> GHHHHHHMIEWIIRRSVANRFLVLMGALFLSIWGTWTIINTPVDALPDLSDVQVIIKTSYPGQAPQIVENQVTYPLTTTMLSVPGAKTVRGFSQFGDSYVYVIFEDGTDPYWARSRVLEYLNQVQGKLPAGVSAELGPDATGVGWIYEYALVDRSGKHDLADLRSLQDWFLKYELKTIPDVAEVASVGGVVKEYQVVIDPQRLAQYGISLAEVKSALDASNQEAGGSSIELAEAEYMVRASGYLQTLDDFNHIVLKASENGVPVYLRDVAKVQIGPEMRRGIAELNGEGEVAGGVVILRSGKNAREVIAAVKDKLETLKSSLPEGVEIVTTYDRSQLIDRAIDNLSGKLLEEFIVVAVVCALFLWHVRSALVAIISLPLGLCIAFIVMHFQGLNANIMSLGGIAIAVGAMVDAAIVMIENAHKRLEEWQHQHPDATLDNKTRWQVITDASVEVGPALFISLLIITLSFIPIFTLEGQEGRLFGPLAFTKTYAMAGAALLAIVVIPILMGYWIRGKIPPESSNPLNRFLIRVYHPLLLKVLHWPKTTLLVAALSVLTVLWPLNKVGGEFLPQINEGDLLYMPSTLPGISAAEAASMLQKTDKLIMSVPEVARVFGKTGKAETATDSAPLEMVETTIQLKPQEQWRPGMTMDKIIEELDNTVRLPGLANLWVPPIRNRIDMLSTGIKSPIGIKVSGTVLADIDAMAEQIEEVARTVPGVASALAERLEGGRYINVEINREKAARYGMTVADVQLFVTSAVGGAMVGETVEGIARYPINLRYPQSWRDSPQALRQLPILTPMKQQITLADVADIKVSTGPSMLKTENARPTSWIYIDA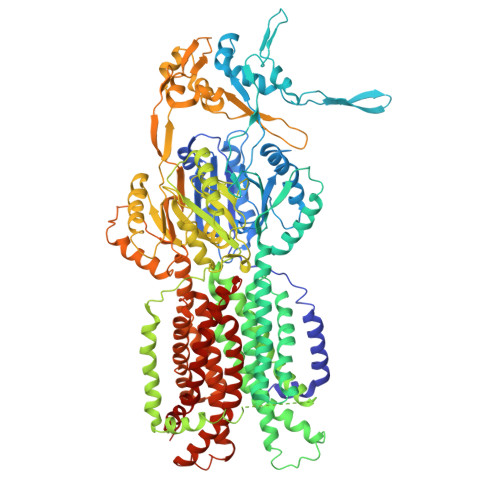RDRDMVSVVHDLQKAIAEKVQLKPGTSVAFSGQFELLERANHKLKLMVPMTLMIIFVLLYLAFRRVGEALLIISSVPFALVGGIWLLWWMGFHLSVATGTGFIALAGVAAEFGVVMLMYLRHAIEAVPSLNNPQTFSEQKLDEALYHGAVLRVRPKAMTVAVIIAGLLPILWGTGAGSEVMSRIAAPMIGGMITAPLLSLFIIPAAYKLMWLHRHRVRK Most pathogenic Gram-negative bacteria transport haem across the plasma membrane using an ATP-dependent active transport system, the ATP-binding cassette (ABC) transporter system. Here we describe the structures of the type II haem importer system (BhuUV-T) from the Gram-negative pathogen Burkholderia cenocepacia. BhuUV-T is a close orthologue of HmuUV-T910, which is a complex of BhuU (TMD), BhuV (NBD) and BhuT (PBP). We successfully characterized the structures of the ABC haem importer, the Bhu system from Burkholderia cenocepacia, and showed that both BhuUV-T and BhuUV adopt an inward-facing conformation in which the periplasmic gate of the haem-translocating channel is closed and the cytoplasmic gate is open.

The crystal structures of BhuUV-T and BhuUV were determined in the nucleotide-free form at 3.2 and 2.8 Å resolution, respectively. The structure of the BhuUV-T complex revealed that BhuT interacts with the periplasmic surface of BhuU. In this interaction, the α3–α4 helices of the N-terminal domain and the α9–α10 helices and a portion of the β-strands of the C-terminal domain of BhuT are bound into a shallow pocket on the periplasmic surface of the BhuU dimer. This binding is mediated by van der Waals contacts, as well as salt bridges between E94 or E231 of BhuT with R84 of BhuU. Most of the space in the cleft of the BhuUV-T complex is occupied by the two H5a helices of the BhuU dimer, and only a very small space is left between BhuT and BhuUV. The structure suggests that the release of haem from the BhuT cleft is facilitated on formation of the BhuUV-T complex and that haem cannot bind into this cleft from the outside of the complex. We prepared haem-loaded BhuT and mixed it with the bacterial ABC haem importer BhuUV to crystallize the haem importer complex BhuUV-T. However, the obtained crystals did not contain haem as judged by the colour of the crystal and the electron density. The structure of BhuUV-T in the haem- and nucleotide-free form was a symmetric dimer containing the inward-facing conformation of BhuU. On the basis of the crystal structure of BhuUV-T determined in this study, the periplasmic gate is tightly sealed by the R204-D200 salt bridges and hydrophobic interaction (L203–L203′) in H5a.

>MGHHHHHHHHHHSSGHIDDDDKHMPAHASPFNAPSSASRAGAARLGTSRRFAPFVLAALAILMGAMSVVALCVGAYRIPLAEAWAALSGDPAAQQARAVLLDIRAPRVVLALLVGGGFGATGAAMQALFRNPLADPGLVGVSSGAALGATTLIVLGPALFAAHASAAALPVAAFAGGLAVAALVYRLAASRGRLALPLLLLAGIAINALVGAAIGLLTFVADDAQLRSLTFWSLGSLGGAQWPTLAAVAPCVALGGVLLVRERDALNALQLGETEALHLGVPVQRLKRRVLVAVALAVGALVSCAGIIGFIGLVAPHCVRLACGPDQRIVLPGAALLGALLTLAADLAARTVAAPADIPLGVLTALLGAPFFLALLWKNRGALGG[2x];>[2x]MLTAHHLDVARRHGTILRDLSLSIEPGRVTALLGRNGAGKSTLLKTFAGELTGSVAPHGVRVTGDVTLNGEPLARIDAPRLACLRAVLPQAAQPAFPFSVDEIVLLGRYPHARRSGATSHRDRDIAWRALERAGADALVGRDVTTLSGGELARVQFARVLAQLWPDHDTTEPGPRYLLLDEPTAALDLAHQHRLLDTVRAVAREWQLGVLAIVHDPNLAARHADAIAMLADGTIVAHGAPRDVMTPAHIAQCYGFAVKMVETGDGTPPVMVPA;> GPLGSKRVIVIGGALAETAFALGGAETPRYRLVGADTTCTYPDAAKRLPKVGYQRALSAEGLLSLRPDLVLASAEAGPPTAIAQVKGAGVTVTTFDERHDVESVRAKITGVAQALDVRDAGAALLQRFDRDWQAARDAVAARVPGGAQPPRVLFVLNHTGTQALVAGQRTAADAMIRYAGARNAMQGFDHYKPLTTEALAAAAPDVVLISDEGLAAVGGHAALLATPGFGATPAGRARRVVSLDALFLLGFGPRLPLAVTTLHRRLSDALA> MSEVVKKFMYLNRKAPYGTIYAWEALEVVLIGAAFDQDVCVLFLDDGVYQLTRGQDTKGIGMKNFSPTYRTLGDYEVRRIYVDRDSLEARGLTQDDLVEIAFEDMETEEEFDNIVEVIDSARVSE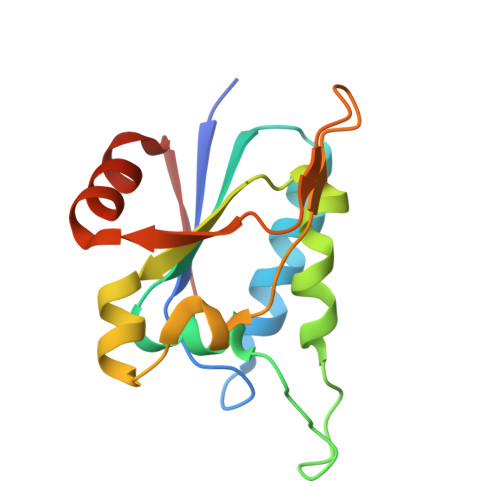LMNESDAVFSF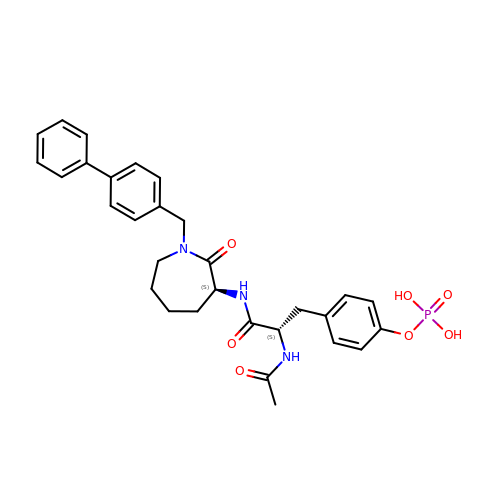N-ACETYL-N-[1-(1,1'-BIPHENYL-4-YLMETHYL)-2-OXOAZEPAN-3-YL]-O-PHOSPHONOTYROSINAMIDE | C30 H34 N3 O7 P | GGPXNASQNUOIPB-NSOVKSMOSA-N> MAAQPLYMEGMASTHQANCIFGEHAGSQCLSNCVMYLASSYYNSETPLVDRASLDDVLEQGMRLDLLLRKSGMLGFRQYAQLHHIPGFLRTDDWATKIFQSPEFYGLIGQDAAIREPFIESLRSVLSRNYAGTVQYLIIICQSKAGAIVVKDKTYYMFDPHCIPNIPNSPAHVIKTNDVGVLLPYIATHDTEYTGCFLYFIPHDYISPEHYIANHYRTIVFEELHGPRMDISRGVESCSITEITSPSVSPAPSEAPLRRDSTQSQDETRPRRPRVVIPPYDPTDRPRPPHQDRPPEQAAGYGGNKGRGGNKGRGGKTGRGGNEGRGGHQPPDEHQPPHITAEHMDQSDGQGADGDMDSTPANGETSVTETPGPEPNPPARPDREPPPTPPATPGATALLSDLTATRGQKRKFSSLKESYPIDSPPSDDDDVSQPSQQTAPDTEDIWIDDPLTPLYPLTDTPSFDITADVTPDNTHPEKAADGDFTNKTTSTDADRYASASQESLGTLVSPYDFTNLDTLLAELGRLGTAQPIPVIVDRLTSRPFREASALQAMDRILTHVVLEYGLVSGYSTAAPSKCTHVLQFFILWGEKLGIPTEDAKTLLESALEIPAMCEIVQQGRLKEPTFSRHIISKLNPCLESLHATSRQDFKSLIQAFNAEGIRIASRERETSMAELIETITARLKPNFNIVCARQDAQTIQDGVGLLRAEVNKRNAQIAQEAAYFENIITALSTFQPPPQSQQTFEVLPDLKLRTLVEHLTLVEAQVTTQTVESLQAYLQSAATAEHHLTNVPNVHSILSNISNTLKVIDYVIPKFIINTDTLAPYKQQFSYLGGELASMFSLDWPHAPAEAVEPLPVLTSLRGKIAEALTRQENKNAVDQILTDAEGLLKNITDPNGAHFHAQAVSIPVLENYVHNAGVLLKGEKSERFSRLKTAIQNLVSSESFITVTLHSTNLGNLVTNVPKLGEAFTGGPHLLTSPSVRQSLSTLCTTLLRDALDALEKKDPALLGEGTTLALETLLGYGSVQDYKETVQIISSLVGIQKLVRDQGADKWATAVTRLTDLKSTLATTAIETATKRKLYRLIQRDLKEAQKHETNRAMEEWKQKVLALDNASPERVATLLQQAPTAKAREFAEKHFKILLPVPADAPVQASPTPMEYSASPLPDPKDIDRATSIHGEQAWKKIQQAFKDFNFAVLRPADWDALAAEYQRRGSPLPAAVGPALSGFLETILGTLNDIYMDKLRSFLPDAQPFQAPPFDWLTPYQDQVSFFLRTIGLPLVRALADKISVQALRLSHALQSGDLQQATVGTPLELPATEYARIASNMKSVFNDHGLQVRSEVADYVEAQRADAHTPHVPRPKIQAPKTLIPHPDAIVADGLPAFLKTSLLQQEAKLLALQRADFESLESDMRAAEAQRKASREETQRKMAHAITQLLQQAPSAISGRPLSLQDPVGFLEGIIYDKVLERESYETGLEGLSWLEQTIKSITVYAPVEEKQRMHVLLDEVKKQRANTETALELEAAATHGDDARLLQRAVDELSPLRVKGGKAAVESWRQKIQTLKSLVQEAEQAGLLLATIDTVAGQAQETISPSTLQGLYQQGQEAMAAIKRFRDSPQLAGLQEKLAELQQYVKYKKQYLEHFEATQSVVFTAFPLTQEVTIPALHYAGPFDNLERLSRYLHIGQTQPAPGQWLLTLPTFDPTRPACVPAGGHEPPLHRQVVFSSFLEAQIRLALSVAGPVPGRGLPGTPQIRRGVEAAACFLHQWDEISRLLP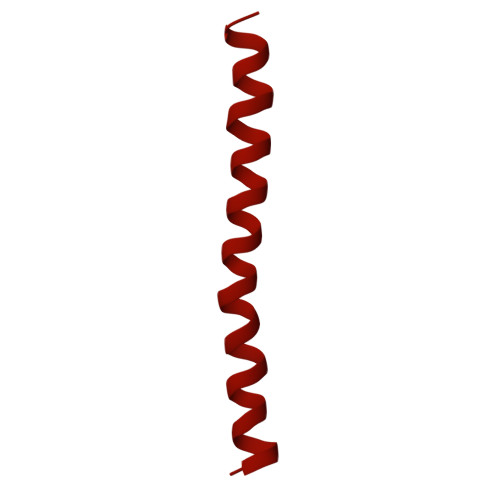EVLDTFFHNAPLPAESSSNAFLAMCVLTHLVYLAGRAVLGPREPEHAAPDAYPREVALAPRDLTYLLLAMWPSWISAILKQPSHAEAAHACLVTLPTMLKAVPYLTLEASAGPLPADMRHFATPEARLFFPARWHHVNVQEKLWLRNDFMSLCHRSPGRARIAVLVWAVTCLDPEVIRQLWSTLRPLTADESDTASGLLRVLVEMEFGPPPKTPRREAVAPGATLPPYPYGLATGERLVGQAQERSGGAGKMPVSGFEIVLGALLFRAPLRIFSTASTHRISDFEGGFQILTPLLDCCPDREPFASLAAAPRRTVPLGDPCANIHTPEEIQIFARQAAWLQYTFANYQIPSTDNPIPIVVLNANNNLENSYIPRDRKADPLRPFYVVPLKPQGRWPEIMTTATTPCRLPTSPEEAGSQFARLLQSQVSATWSDIFSRVPERLAPNATQKSSQTMSEIHEVAATPPLTITPNKPTGTPHVSPEADPITERKRGQQPKIVADNMPSRILPSLPTPKPREPRITLPHALPVISPPAHRPSPIPHLPAPQVTEPKGVLQSKRGTLVLRPAAVIDPRKPVSAPITRYERTALQPPRTEGEGRRPPDTQPVTLTFRLPPTAPTPATAALETKTTPPSTPPHAIDISPPQTPPMSTSPHARDTSPPAEKRAAPVIRVMAPTQPSGEARVKRVEIEQGLSTRNEAPPLERSNHAVPAVTPRRTVAREIRIPPEIKAGWDTAPDIPLPHSSPESSPPTSPQPIRVDDKSPLPNLVERYARGFLDTPSVEVMSLENQDIAVDPGLLTRRIPSVVPMPHPIMWSPIVPISLQNTDIDTAKITLISFIRRIKQKVAALSASLAETVDRIKKWYL3-[(4S)-6-CHLORO-2-METHYL-4-(4-METHYLPHENYL)QUINAZOLIN-3(4H)-YL]-N,N-DIMETHYLPROPAN-1-AMINE 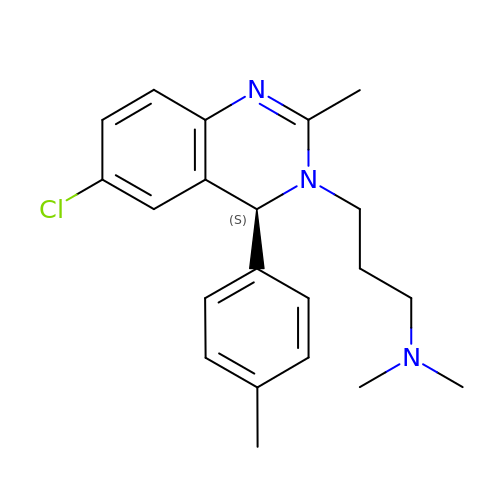| C21 H26 Cl N3 | RZVYHDCYMAMDJY-NRFANRHFSA-N> TGGRNSIRYSELAPLFDT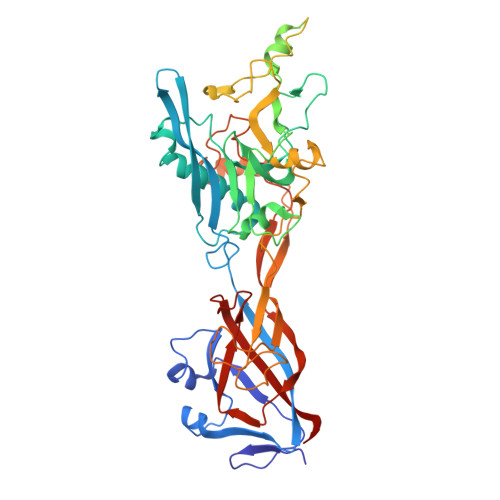TRVYLVDNKSTDVASLNYQNDHSNFLTTVIQNNDYSPGEASTQTINLDDRSHWGGDLKTILHTNMPNVNEFMFTNKFKARVMVSRSLTKDKQVELKYEWVEFTLPEGNYSETMTIDLMNNAIVEHYLKVGRQNGVLESDIGVKFDTRNFRLGFDPVTGLVMPGVYTNEAFHPDIILLPGCGVDFTHSRLSNLLGIRKRQPFQEGFRITYDDLEGGNIPALLDVDAYQASLKDDTEQGGDGAGGGNNSGSGAEENSNAAAAAMQPVEDMNDHAIRGDTFATRAEEKRAEAEAAAEAAAPAAQPEVEKPQKKPVIKPLTEDSKKRSYNLISNDSTFTQYRSWYLAYNYGDPQTGIRSWTLLCTPDVTCGSEQVYWSLPDMMQDPVTFRSTSQISNFPVVGAELLPVHSKSFYNDQAVYSQLIRQFTSLTHVFNRFPENQILARPPAPTITTVSENVPALTDHGTLPLRNSIGGVQRVTITDARRRTCPYVYKALGIVSPRVLSSRTF> VNYAAGLSPYADKGKCGLPEIFDPPEELERKVWELARLVWQSSSVVFHTGAGISTASGIPDFRGPHGVWTMEERGLAPKFDTTFESARPTQTHMALVQLERVGLLRFLVSQNVDG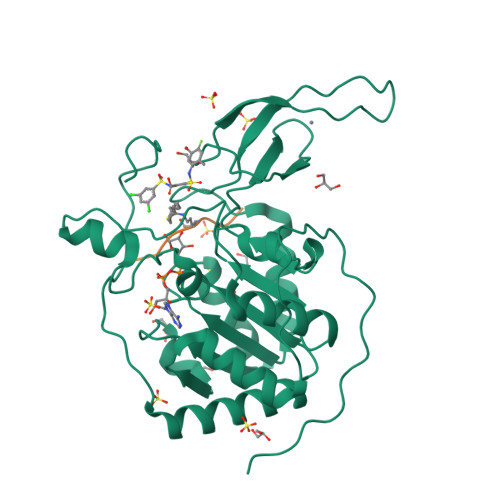LHVRSGFPRDKLAELHGNMFVEECAKCKTQYVRDTVVGTMGLKATGRLCTVAKARGLRACRGELRDTILDWEDSLPDRDLALADEASRNADLSITLGTSLQIRPSGNLPLATKRRGGRLVIVNLQPTKHDRHADLRIHGYVDEVMTRLMKHLGLEIPAWDGPRVLERALPPLPRPPTPKLEPKEESPTRINGSIPAGPKQE;> QTARKSTGG>MSETAGKPIECKAAIAWEAKKPLEVRTVTVAPPGPGEVRVQIKATALCQTDAYTLGGLDPEGRFPCILGHEAAGVVESVGEGVTSVKPGDHVIPCYQAYCGECKFCKHPESNLCVSVRAFTGKGVMKSDGKPRFTVDGKPIYHFMGTSTFSEYTVVHEQSVAKIDVNAPLDKVCLLGCGVSTGWGAVFNTAKVTAGSTVAVFGLGAVGLAVIEAAKRAGASRIIAVDIDPTKFPTAKEFGATDCINPKDHEKPIQQVIVEMTEWGCDYTFECIGNTAVMRAALECAHRGWGTSVIVGVAAAGQEISTRPFQLVTGRRWMGTAFGGYKSRVQVPDLVTDYM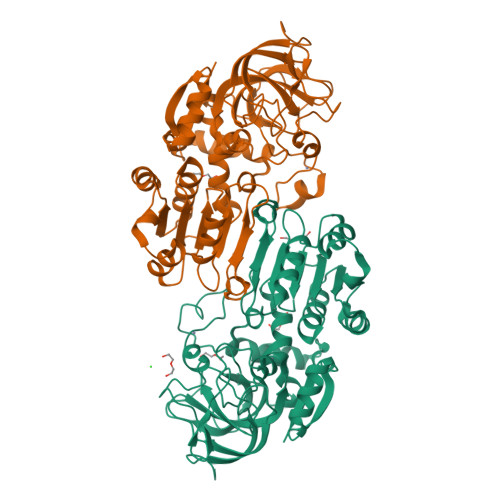SGATLLDKYITHNMKFDQINEAFELLHAGECLRCVLTF[6x]6-BROMO-7-{4-[(5-METHYLISOXAZOL-3-YL)METHYL]PIPERAZIN-1-YL}-2-[4-(4-METHYLPIPERAZIN-1-YL)PHENYL]-1H-IMIDAZO[4,5-B]PYRIDINE | C26 H31 Br N8 O | 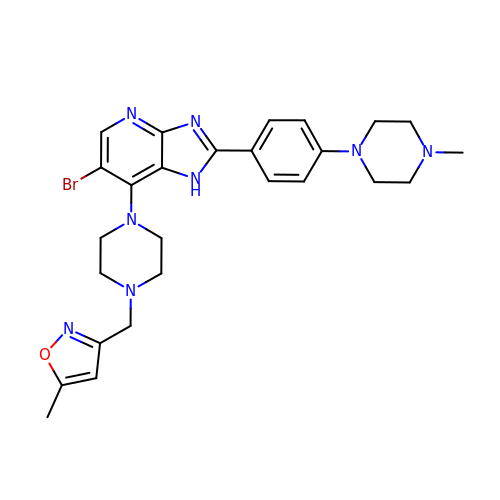GFLQCBTXTRCREJ-UHFFFAOYSA-N>[2x]NLKPVDAMQCFDCHTQIEDMHTVGKHATVNCVHCHDATEHVETASSRRMGERPVTRMDLEACATCHTAQFNSFVEVRHESHPRLEKATPTSRSPMFDKLIAGHGFAFEHAEPRSHAFMLVDHFVVDRAYGGRFQFKNWQKVTDGMGAVRGAWTVLTDADPESSDQRRFLSQTAT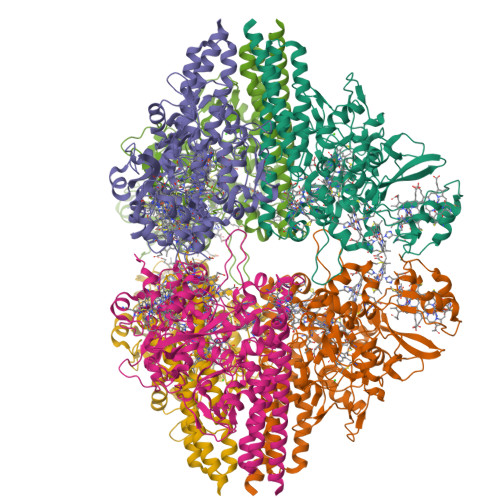AANPVCLNCKTQDHILDWAYMGDEHEAAKWSRTSEVVEFARDLNHPLNCFMCHDPHSAGPRVVRDGLINAVVDRGLGTYPHDPVKSEQQGMTKVTFQRGREDFRAIGLLDTADSNVMCAQCHVEYNCNPGYQLSDGSRVGMDDRRANHFFWANVFDYKEAAQEIDFFDFRHATTGAALPKLQHPEAETFWGSVHERNGVACADCHMPKVQLENGKVYTSHSQRTPRDMMGQACLNCHAEWTEDQALYAIDYIKNYTHGKIVKSEYWLAKMIDLFPVAKRAGVSEDVLNQARELHYDAHLYWEWWTAENSVGFHNPDQARESLMTSISKSKEAVSLLNDAIDAQVAV> MDCAKEGEVCSWGKK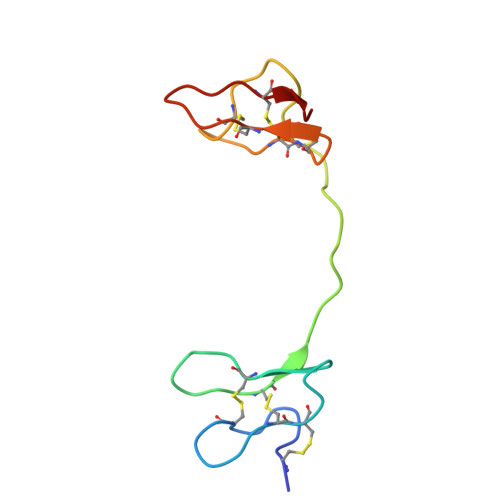CCDLDNFYCPMEFIPHCKKYKPYVPVTTNCAKEGEVCGWGSKCCHGLDCPLAFIPYCEKYR>[2x]MTVPYLNSNRNVASYLQSNSSQEKTLKERFSEIYPIHAQDVRQFVKEHGKTKISDVLLEQVYGGMRGIPGSVWEGSVLDPEDGIRFRGRTIADIQKDLPKAKGSSQPLPEALFWLLLTGEVPTQAQVENLSADLMSRSELPSHVVQLLDNLPKDLHPMAQFSIAVTALESESKFAKAYAQGISKQDYWSYTFEDSLDLLGKLPVI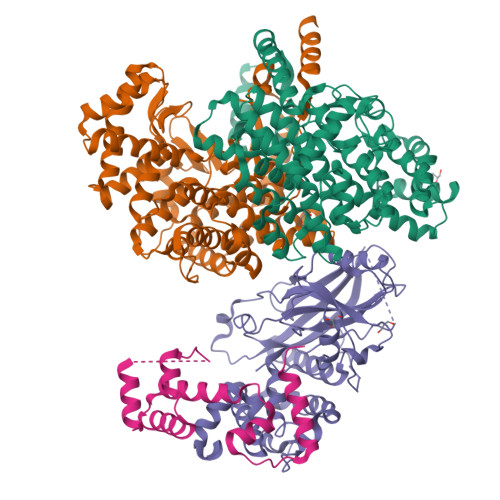AAKIYRNVFKDGKMGEVDPNADYAKNLVNLIGSKDEDFVDLMRLYLTIHSDHEGGNVSAHTSHLVGSALSSPYLSLASGLNGLAGPLHGRANQEVLEWLFALKEEVNDDYSKDTIEKYLWDTLNSGRVIPGYGHAVLRKTDPRYMAQRKFAMDHFPDYELFKLVSSIYEVAPGVLTEHGKTKNPWPNVDAHSGVLLQYYGLKESSFYTVLFGVSRAFGILAQLITDRAIGASIERPKSYSTEKYKELVKNIESKL;> MNQSDSSLMDLPLEIHLSLLEYVPNELRAVNKYFYVLHNHSYKEKSLAWIAEDNYIWAVVKHSLCLYVKSLDPLRQHAREIIQETKEPGFNVPLCMTKYIADSWYIVYNALQYPGKIINMGWDKYTKSQDLNGSDSTSNFNSRPKERTLMQSLTALPVNFWSRKKDEPTPVNVWFYVKNAHVARYIPKIITEIGICNYGPKQIVASAGYINELITSEGIYCVNLGHLPRLYDEQIFEGTGTTHLPLELKAIDRTDSDVCINSDLVLLGYDFIPYQISKPWLLFRIEPVNSIEAIFNYSECSFSYQFAWSLACLQSEEKISFPRDTIIGHGLPYKPSKLIRIFVYKHPEQKQDLGQEIALPNWNTPYLRR;> MVTSNVVLVSGEGERFTVDKKIAERSLLLKNYLNDMHDSNLQNNSDSESDSDSETNHKSKDNNNGDDDDEDDDEIVMPVPNVRSSVLQKVIEWAEHHRDSNFPDEDDDDSRKSAPVDSWDREFLKVDQEMLYEIILAANYLNIKPLLDAGCKVVAEMIRGRSPEEIRRTFNIVNDFTPEEEAAIRRENEWAEDR>[2x]GSFTEELHLIPPLNFSMVDNGIFRSGFPDSANFSFLQTLGLRSIIYLCPEPYPESNLQFLKSNGIRLFQFGIEGNKEPFVNIPDH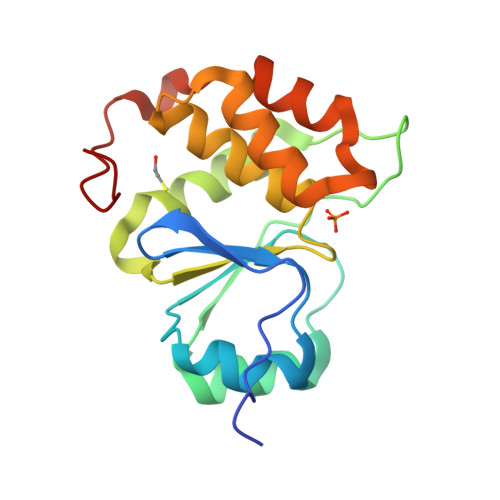KIRMALKVLLDEKNHPVLIHCKRGKHRTGCLVGCLRKLQKWCLTSIFDEYQRFAAAKARVSDQRFMEIFDVSSFSHIPMSFSCSIR> HHHHHHMATLKRDKGLDNTLKVLKQGYLYTTNQRNRLNTSVFQTKALGGKPFVVVTGKEGAEMFYNNDVVQREGMLPKRIVNTLFGKGAIQTVDGKKHVDR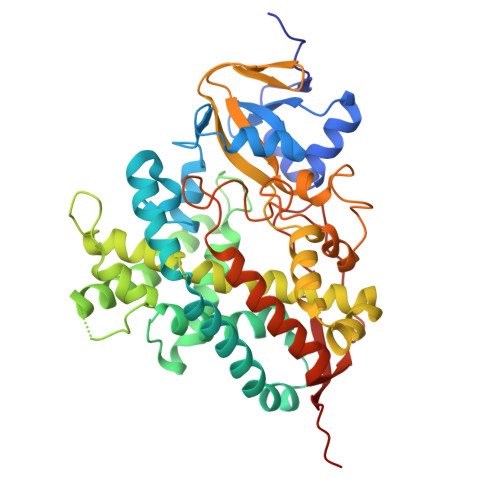KALFMSLMTEGNLNYVRELTRTLWHANTQRMESMDEVNIYRESIVLLTKVGTRWAGVQAPPEDIERIATDMDIMIDSFRALGGAFKGYKASKEARRRVEDWLEEQIIETRKGNIHPPEGTALYEFAHWEDYLGNPMDSRTCAIDLMNTFRPLIAINRFVSFGLHAMNENPITREKIKSEPDYAYKFAQEVRRYYPFVPFLPGKAKVDIDFQGVTIPAGVGLALDVYGTTHDESLWDDPNEFRPERFETWDGSPFDLIPQGGGDYWTNHRCAGEWITVIIMEETMKYFAEKITYDVPEQDLEVDLNSIPGYVKSGFVIKNVREVVDRT> GMSSVTWAPGNYPSTRRSDHVDTYQSASKGEVPVPDPYQWLEESTDEVDKWTTAQADLAQSYLDQNADIQKLAEKFRASRNYAKFSAPTLLDDGHWYWFYNRGLQSQSVLYRSKEPALPDFSKGDDNVGDVFFDPNVLAADGSAGMVLCKFSPDGKFFAYAVSHLGGDYSTIYVRSTSSPLSQASVAQGVDGRLSDEVKWFKFSTIIWTKDSKGFLYQRYPARERHEGTRSDRNAMMCYHKVGTTQEEDIIVYQDNEHPEWIYGADTSEDGKYLYLYQFKDTSKKNLLWVAELDEDGVKSGIHWRKVVNEYAADYNIITNHGSLVYIKTNLNAPQYKVITIDLSKDEPEIRDFIPEEKDAKLAQVNCANEEYFVAIYKRNVKDEIYLYSKAGVQLTRLAPDFVGAASIANRQKQTH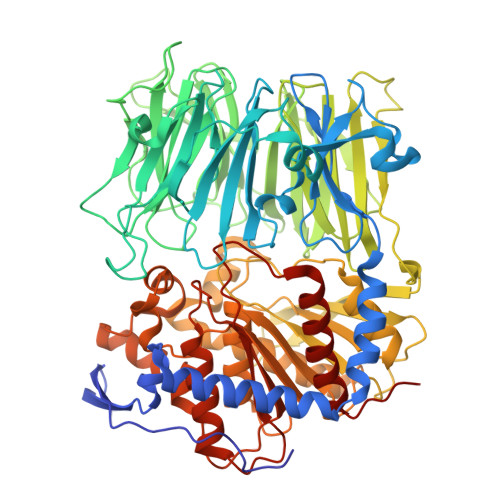FFLTLSGFNTPGTIARYDFTAPETQRFSILRTTKVNELDPDDFESTQVWYESKDGTKIPMFIVRHKSTKFDGTAAAIQYGYGGFATSADPFFSPIILTFLQTYGAIFAVPSIRGGGEFGEEWHKGGRRETKVNTFDDFIAAAQFLVKNKYAAPGKVAINGAANGGLLVMGSIVRAPEGTFGAAVPEGGVADLLKFHKFTGGQAWISEYGNPSIPEEFDYIYPLSPVHNVRTDKVMPATLITVNIGDGRVVPMHSFKFIATLQHNVPQNPHPLLIKIDKSWLGHGMGKPTDKNVKDAADKWGFIARALGLELKTVE> MKLKLIVNGCEAPDDYKLLRTTINTVASLRKTAILRFNSERLTIISTPKSSLNSSNNGTILRGDTGQLWCTIPHDVFRLYTVISARELNTITMECNCDSLLSVFKRYDRVMNQGSSSNMTIKLQSMPEWNTNNGTLSGGTAGGVDTTSKPNPICALGITFEEIVHTSGPNDAIVMNGGVDEHNGLPTTVGTGNLLASNKVIMHSFKVPVKLLFRAQDTRIQEPMINYIQLMMYKLPPISGEFGSAFHGFIRRVERYSNVNHIHLMGVKKKEHGNEGDDVELKIIVNELDWHLEICWNGPLDSVIQRQEGLTDNPSQNQHIDTDGRQEEGSLPIIEADKPMSSLYTNTRDREMEENIRYDEDLLRIEDSSIADTRGNIYTADTSGD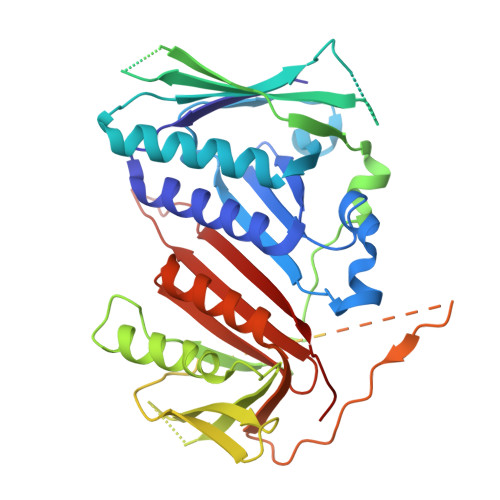TEFNDISVMVEKAEQESSSTHEVIIRCKDWKVCSKLYAAFEEVVLAISHDESCVFHCSLDRGSLEDSEDVEKPRERGQIIYYIARSKGL> VIHVTKEVKEVATLSCGHNVSVEELAQTRIYWQKEKKMVLTMMSGDMNIWPEYKNRTIFDITNNLSIVILALRPSDEGTYECVVLKYEKDAFKREHLAEVTLSVKADFPTPSISDFEIPTSNIRRIICSTSGGFPEPHLSWLENGEELNAINTTVSQDPETELYAVSSKLDFNMTTNHSFMCLI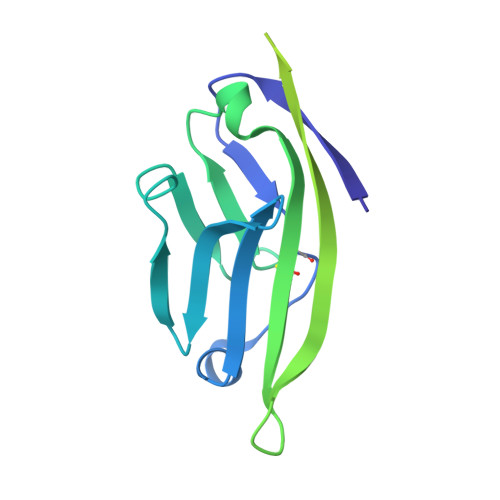KYGHLRVNQTFNWNTT> MGWCVMAVLVDSETRVLVQGITGREGSFHAKAMLEYGTKVVAGVTPGKGGSEVHGVPVYDSVKEALAEHPEINTSIVF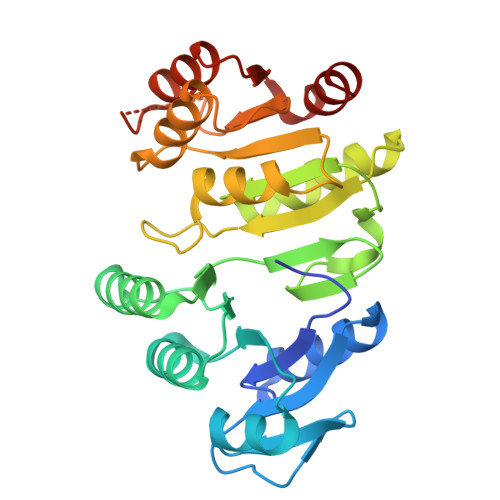VPAPFAPDAVYEAVDAGIRLVVVITEGIPVHDTMRFVNYARQKGATIIGPNCPGAITPGQAKVGIMPGHIFKEGGVAVVSRSGTLTYEISYMLTRQGIGQSTVIGIGGDPIVGLSFTEALKLFQEDPQTEALVLIGEIGGDMEERAAEMIKKGEFTKPVIAYIAGRTAPPEKRMGHAGAIIMMGTGTYEGKVKALREAGVEVAETPFEVPELVRKALRR2-deoxy-2-fluoro-alpha-D-glucopyranuronic acid | C6 H9 F O6 | 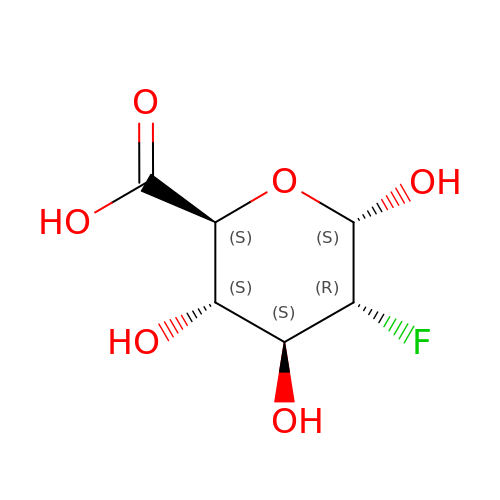LDVYRSUUUDDWHG-CLQWQSTFSA-N Internal thioester bonds are formed between the side chains of Cys and Gln residues, most likely self-generated by a favorable environment during protein folding. Here we experimentally demonstrate that thioester domains are prevalent in Gram-positive surface proteins, and that they share a conserved three-dimensional structure despite being divergent in protein sequence. This suggests that thioester domains may target distinct receptors and have a widespread but currently unappreciated role in mediating pathogen adhesion to hosts. Putative TEDs appear in a variety of domain architectures, but are almost always located at the N-termini of proteins containing secretion signals and C-terminal LPXTG cell wall-anchoring motifs.

Further, we present the identification of host fibrinogen as a covalently bound target of the streptococcal surface protein SfbI. In a thioester-dependent mechanism, SfbI reacts with one specific lysine residue in fibrinogen, forming a very stable intermolecular amide bond. Using a combination of computational, biochemical, structural and cell-based assays we reveal a novel mechanism for host adhesion mediated by a pathogen-encoded covalent interaction.

>GPDEKTVPNFKSPDPDYPWYGYDSYRGIFARYHNLKVNLKGSKEYQAYCFNLTKYFPRPTYSTTNNFYKKIDGSGSAFKSYAANPRVLDENLDKLEKNILNVIYNGYKSNANGFMNGIEDLNAILVTQNAIWYYSDSAPLNDVNKMWEREVRNGEISESQVTLMREALKKLIDPNLEATAANKIPSGYRLNIFKSENEDYQNLLSAEYVP[2x]>[3x]GSQDSTSDLIPAPPLSKVPLQQNFQDNQFQGKWYVVGLAGNAILREDKDP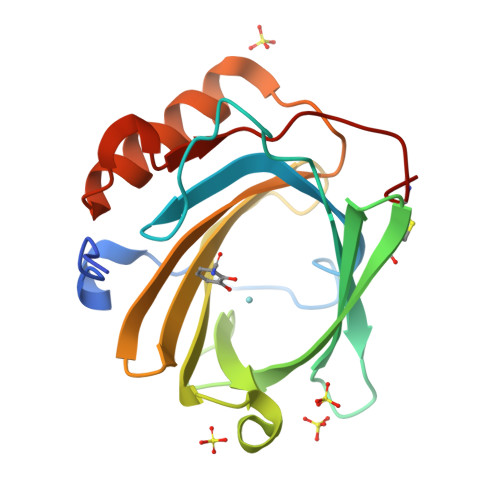QKMYATIYELKEDKSYNVTSVLFRKKKCDYWIRTFVPGSQPGEFTLGNIKSYPGLTSYLVRVVSTNYNQHAMVFFKKVSQNREYFKITLYGRTKELTSELKENFIRFSKSLGLPENHIVFPVPIDQCIDG>MGNKLFVLDLGEIRVDENFIIANSTFVTPQKPTVSSRLIDIPVSAYLIQCTDATVLYDTGCHPECMGTNGRWPAQSQLNAPYIGASECNLPERLRQLGLSPDDISTVVLSHLHNDHAGCVEYFGKSRLIAHEDEFATAVRYFATGDHSSPYIVKDIEAWLATPRNWDLVGRDERERELAPGVNLLNFGTGHASGMLGLAVRLEKQPGFLLVSDACYTATNYGPPARRAGVLHDTIGYDRTVSHIRQYAESRS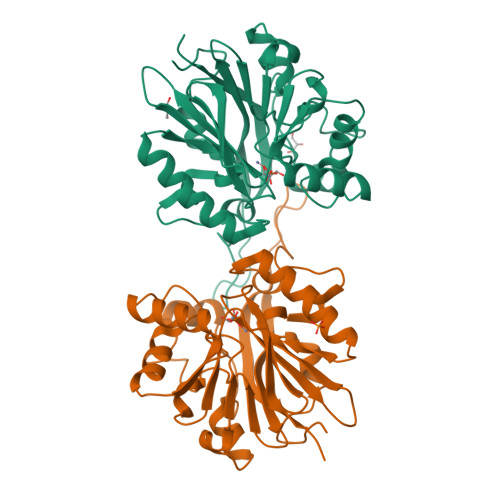LTVLFGHDREQFASLIKSTDGFYE[6x]>MVLDLDLFRVDKGGDPALIRETQEKRFKDPGLVDQLVKADSEWRRCRFRADNLNKLKNLCSKTIGEKMKKKEPVGDDESVPENVLSFDDLTADALANLKVSQIKKVRLLIDEAILKCDAERIKLEAERFENLREIGNLLHPSVPISNDEDVDNKVTSIWGDCTVRKKYSHVDLVVMVDGFEGEKGAVVAGSRGYFLKGVLVFLEQALIQYALRTLGSRGYIPIYTPFFMRKEVMQEVAQLSQFDEELYKVIGKGSEKSDDNSYDEKYLIATSEQPIAALHRDEWLRPEDLPIKYAGLSTCFRQEVGSHGRDTRGIFRVHQFEKIEQFVYSSPHDNKSWEMFEEMITTAEEFYQSLGIPYHIVNIVSGSLNHAASKKLDLEAWFPGSGAFRELVSCSNCTDYQARRLRIRYGQTKKMMDKVEFVH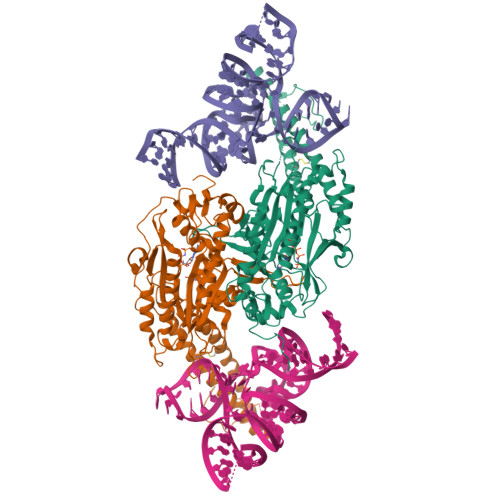MLNATMCATTRTICAILENYQTEKGITVPEKLKEFMPPGLQELIPFVKPAPIEQEPSKKQKKQHEGSKKKAAARDVTLENRLQNMEVTDALEHHHHHH[2x]>[3x]MATPHINA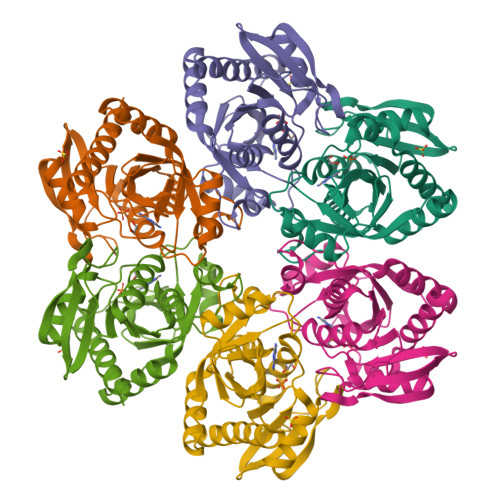EMGDFADVVLMPGDPLRAKYIAETFLEDAREVNNVRGMLGFTGTYKGRKISVMGHGMGIPSCSIYTKELITDFGVKKIIRVGSCGAVLPHVKLRDVVIGMGACTDSKVNRIRFKDHDFAAIADFDMVRNAVDAAKALGIDARVGNLFSADLFYSPDGEMFDVMEKYGILGVEMEAAGIYGVAAEFGAKALTICTVSDHIRTHEQTTAAERQTTFNDMIKIALESVLLGDKE> MFKVYGYDSNIHKCGPCDNAKRLLTVKKQPFEFINIMPEK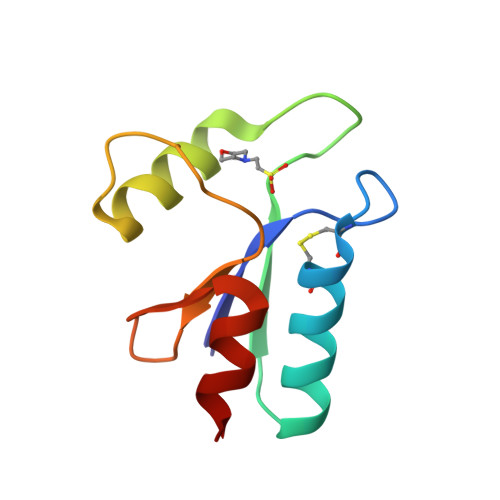GVFDDEKIAELLTKLGRDTQIGLTMPQVFAPDGSHIGGFDQLREYFK Respiratory chains are crucial for cellular energy conversion and consist of multi‐subunit complexes that can assemble into supercomplexes. In mammalian cells, the mitochondrial respiratory chain (MRC) is formed by four distinct complexes (CI–CIV) (Lobo‐Jarne & Ugalde, 2018). Together with the ATP synthase (CV), these complexes form the oxidative phosphorylation (OXPHOS) system, in which electron transfer to molecular oxygen is coupled with the formation of an electrochemical gradient over the inner mitochondrial membrane to drive ATP synthesis. Three major models have been proposed for the structural organization of the MRC: the solid‐state, the liquid‐state (fluid), and the plasticity model (Acín‐Pérez et al, 2008; Milenkovic et al, 2017; Lobo‐Jarne & Ugalde, 2018). The latter consolidates the previous two models and is based on findings from the past two decades, showing that MRC complexes are not randomly distributed within the inner mitochondrial membrane, but can be assembled into supramolecular structures termed supercomplexes (SCs). In summary, our results demonstrate that the formation of SCs is important for efficient electron transfer between CIII and CIV by positioning the Cyt c binding sites of both complexes in close vicinity, a conserved feature of SC architecture found in multiple organisms.

To this end, we improved the resolution of our previous SC structure (Rathore et al, 2019). This yielded a CIII2/CIV density map with an overall resolution of 3.17 Å, and, more importantly, after particle subtraction of CIII2, the CIV density was solved to an overall resolution of 3.41 Å (Fig EV1A–D, Table EV1). Particles from a dataset previously acquired (Rathore et al, 2019) were re‐processed using an updated version of the software cryoSPARC (Punjani et al, 2017) (Fig EV1A; Table EV1). Using the particle subtraction tool and local refinement tool to subtract the signal from CIII2 and refine CIV alone, we could generate a 3.41 Å density map (GSFSC = 0.143; B‐factor: −125.9; Fig EV1B), which was used to model the atoms of CIV. Additional improvement of the CIV subunits was built using the 3.41 Å (FSC = 0.143) density map. A Ribbon diagram of CIV with Cox12, Cox13, and Cox26 annotated. B–D Example densities of Cox12 (B), Cox13 (C), and Cox26 (D) demonstrating parts of the subunits that improved due to the re‐processing of the data set.

> WLYSTNAKDIAVLYFMLAIFSGMAGTAMSLIIRLELAAPGSQYLHGNSQLFNVLVVGHAVLMIFFLVMPALIGGFGNYLLPLMIGATDTAFPRINNIAFWVLPMGLVCLVTSTLVESGAGTGWTVYPPLSSIQAHSGPSVDLAIFALHLTSISSLLGAINFIVTTLNMRTNGMTMHKLPLFVWSIFITAFLLLLSLPVLSAGITMLLLDRNFNTSFFEVSGGGDPILYEHLFWFFGHPEVYILIIPGFGIISHVVSTYSKKPVFGEISMVYAMASIGLLGFLVWSHHMYIVGLDADTRAYFTSATMIIAIPTGIKIFSWLATIHGGSIRLATPMLYAIAFLFLFTMGGLTGVALANASLDVAFHDTYYVVGHFHYVLSMGAIFSLFAGYYYWSPQILGLNYNEKLAQIQFWLIFIGANVIFFPMHFLGINGMPRRIPDYPDAFAGWNYVASIGSFIATLSLFLFIYILYDQLVNGLNNKVNNKSVIYNKAPDFVESNTIFNLNTVKSSSIEFLLTSPPAVHSFNTPAVQS;> DVPTPYACYFQDSATPNQEGILELHDNIMFYLLVILGLVSWMLYTIVMTYSKNPIAYKYIKHGQTIEVIWTIFPAVILLIIAFPSFILLYLCDEVISPAMTIKAIGYQWYWKYEYSDFINDSGETVEFESYVIPDELLEEGQLRLLDTDTSMVVPVDTHIRFVVTAADVIHDFAIPSLGIKVDATPGRLNQVSALIQREGVFYGACSELCGTGHANMPIKIEAVSLPKFLEWLNEQ;> THLERSRHQQHPFHMVMPSPWPIVVSFALLSLALSTALTMHGYIGNMNMVYLALFVLLTSSILWFRDIVAEATYLGDHTMAVRKGINLGFLMFVLSEVLIFAGLFWAYFHSAMSPDVTLGACWPPVGIEAVQPTELPLLNTIILLSSGATVTYSHHALIAGNRNKALSGLLITFWLIVIFVTCQYIEYTNAAFTISDGVYGSVFYAGTGLHFLHMVMLAAMLGVNYWRMRNYHLTAGHHVGYETTIIYTHVLDVIWLFLYVVFYWWGV;> VVKTAQNLAEVNGPETLIGPGAKEGTVPTDLDQETGLARLELLGKLEGIDVFDTKPLDSSRKGTMKDPIIIESYDDYRYVGCTGSPAGSHTIMWLKPTVNEVARCWECGSVYKLNPV;> ALSNAAVMDLQSRWENMPSTEQQDIVSKLSERQKLPWAQLTEPEKQAVWYISYGEWGPRRPVLNKGDSSFIAKGVAAGLLFSVGLFAVVRMAGGQDAKTMNKEWQLKSDEYLKSKNANPWGGYSQVQS;> ETFEEFTARYEKEFDEAYDLFEVQRVLNNCFSYDLVPAPAVIEKALRAARRVNDLPTAIRVFEALKYKVENEDQYKAYLDELKDVRQELGVPLKEELFP;> NKVIQLQKIFQSSTKPLWWRHPRSALYLYPFYAIFAVAVVTPLLYIPNAIRGIKA;> VHFKDGVYENIPFKVKGRKTPYALSHFGFFAIGFAVPFVACYVQLKKSGAF;> TIAPITGTIKRRVIMDIVLGFSLGGVMASYWWWGFHMDKINKREKFYAELAE;> NSPLHTVGFDARFPQQNQTKHCWQSYVDYHKCVNMKGEDFAPCKVFWKTYNALCPLDWIEKWDDQREKGIFAGDINSD;> NALKPAFGPPDKVAAQKFKESLMATEKHAKDTSNMWVKISVWVALPAIALTAVNTYFVEKEHAEHREHLKHVPDSEWPRDYEFMNIRSKPFFWGDGDKTLFWNPVVNRHIEHDD;> ESWVITEGRRLIPEIFQWSAVLSVCLGWPGAVYFFSKA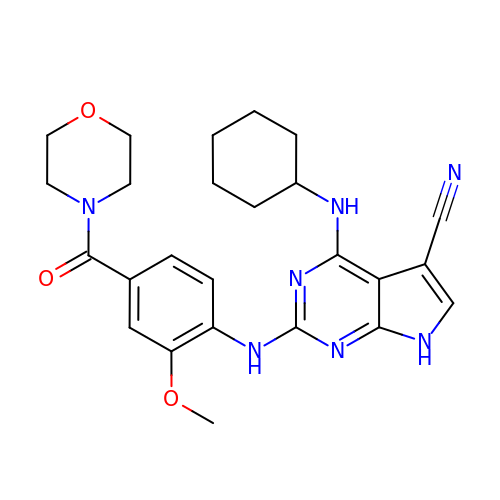4-(cyclohexylamino)-2-[(2-methoxy-4-morpholin-4-ylcarbonyl-phenyl)amino]-7H-pyrrolo[2,3-d]pyrimidine-5-carbonitrile | C25 H29 N7 O3 | IOKQAXDJAARNRZ-UHFFFAOYSA-N>MTTQPQLKENLTQWEYLALNSELNIADGHARQALSPGQQKIVNELPVLWAESEQRPVQQIESEAHQAYFTLLGQHGYPAEPGRVLSCYSSSVSMEILARSLSASVDRVALVHPTFDNIADLLRGNGLDLVPVEEDALHGADLSAELLSSVGCVFVTTPNNPTGRVLAEERLRRLAEQCAEHGTVLALDTSFRGFDAAAHYDHYAVLQEAGCRWVVIEDTGKLWPTLDLKAGLLVFSEDIGLPVEKIYSDILLGVSPLILALIREFSRDAADGGLADLHAFILHNRSVVRRALAGVEGVSFPDPESRSSVERVAFAGRTGTEVWEELQRHHVFALPCRQFHWAEPSDGDHMVRIALSRSTEPLEKS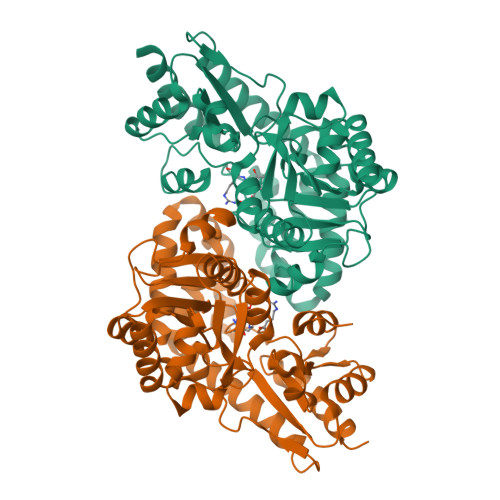VQVLRTVLETR[4x]> GSEMELEIDRNLDQIQQVSNRLKKMALTTGKELDSQQKRLN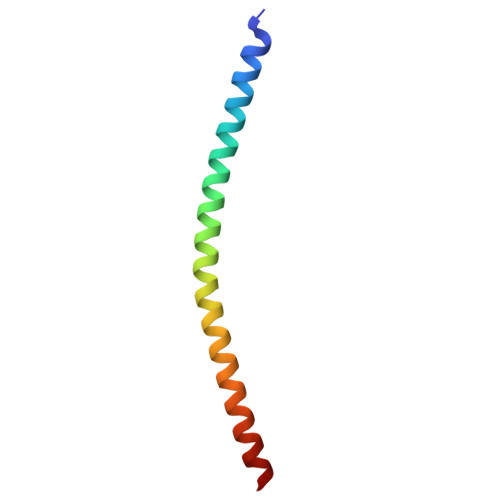NIEESTDDLDINLHMNTNRLAGI> MDFGSLETVVANSAFIAARGSFDASSGPASRDRKYLARLKLPPLSKCEALRESLDLGFEGMCLEQPIGKRLFQQFLRTHEQHGPALQLWKDIEDYDTADDALRPQKAQALRAAYLEPQAQLFCSFLDAETVARARAGAGDGLFQPLLRAVLAHLGQAPFQEFLDSLYFLRFLQWKWLEAQPMGEDWFLDFRVLGRGGFGEVFACQMKATGKLYACKKLNKKRLKKRKGYQGAMVEKKILAKVHSRFIVSLAYAFETKTDLCLVMTIMNGGDI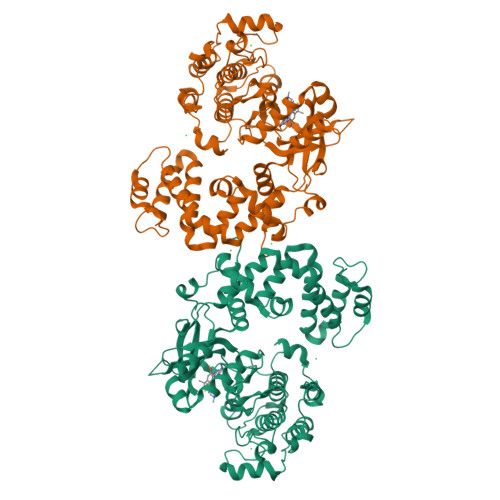RYHIYNVDEDNPGFQEPRAIFYTAQIVSGLEHLHQRNIIYRDLKPENVLLDDDGNVRISDLGLAVELKAGQTKTKGYAGTPGFMAPELLLGEEYDFSVDYFALGVTLYEMIAARGPFRARGEKVENKELKQRVLEQAVTYPDKFSPASKDFCEALLQKDPEKRLGFRDGSCDGLRTHPLFRDISWRQLEAGMLTPPFVPDSRTVYAKNIQDVGAFSTVKGVAFEKADTEFFQEFASGTCPIPWQEEMIETGVFGDLNVWRPDGQMPDDMKGVSGQEAAPSSKSGMCVLS> MKQYLELMQKVLDEGTQKNDRTGTGTLSIFGHQMRFNLQDGFPLVTTKRCHLRSIIHE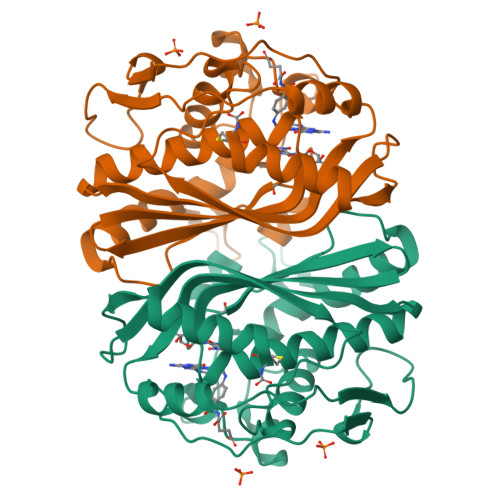LLWFLQGDTNIAYLHENNVTIWDEWADENGDLGPVYGKQWRAWPTPDGRHIDQITTVLNQLKNDPDSRRIIVSAWNVGELDKMALAPCHAFFQFYVADGKLSCQLYQRSCDVFLGLPFNIASYALLVHMMAQQCDLEVGDFVWTGGDTHLYSNHMDQTHLQLSREPRPLPKLIIKRKPESIFDYRFEDFEIEGYDPHPGIKAPVAI> MSKNRSSLQSGPLNSELLEEQKQEIYEAFS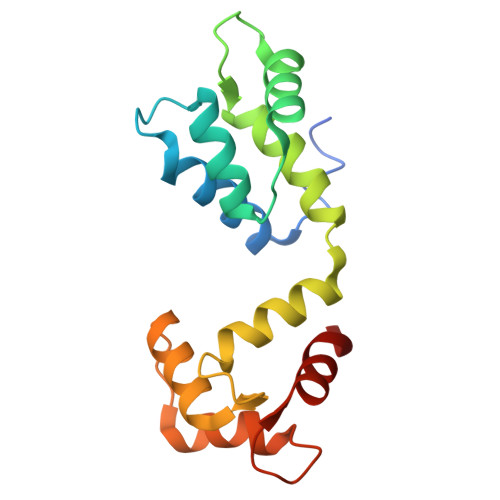LFDMNNDGFLDYHELKVAMKALGFELPKREILDLIDEYDSEGRHLMKYDDFYIVMGEKILKRDPLDEIKRAFQLFDDDHTGKISIKNLRRVAKELGETLTDEELRAMIEEFDLDGDGEINENEFIAICTDS>[2x]GSYDSSSSSSNDSSARNEEDESCMFALKLLGGFAVPFTIKAVIELGVMDQLLTAERAMSAEELVAAAVAAQLPRPEVACTMVDRLLRFLASHSVVRCTTEVVVGTDDATTTTCCRRSYAASPVCKWFARNGVEDSVLPLGMMILNKTFLDSWQNITDAVLEGAAPFEKTYGMPMFEYLSTNGPLNTVFHEAMANHSMIITKKLLKFFRGFEGLDVLVDVGGGNGTTLQMIRGQYKNMRGINYDLPHVIAQAAPVEGVEHVGGSMFDNIPRGNAVLLKWILHDWDDKACIKILKNCYTALHVRGKVIVLEYVVPDEPEPTLAAQGAFELDLTMLVTFGSGKERTQREFSELAMEAGFSREFKATYIFANVWALEFTK

A stilbene O-methyltransferase, SbSOMT, is first shown to be indispensable for pathogen-inducible pterostilbene (3,5-bis-O-methylated) biosynthesis in sorghum (Sorghum bicolor). Phylogenetic analysis indicates the recruitment of genus-specific SOMTs from canonical caffeic acid O-methyltransferases (COMTs) after the divergence of Sorghum spp. from Saccharum spp. In recombinant enzyme assays, SbSOMT and COMTs regioselectively catalyze O-methylation of stilbene A-ring and B-ring respectively. Whilst SbSOMT shows global structural resemblance to SbCOMT, molecular characterizations illustrate two hydrophobic residues (Ile144/Phe337) crucial for substrate binding orientation leading to 3,5-bis-O-methylations in the A-ring. The catalytic residues of SbSOMT are highly conserved with all reported COMTs, including His282 as the key nucleophile, whereas Asp283, Glu310, and Glu342 collectively charge the basicity or confine His282 in its reactive conformation.

To rationalize their different catalytic regioselectivities, structural analyses involving X-ray crystallography and computational methods were conducted. We solved the crystal structure of an SbSOMT-resveratrol-nicotinamide adenine dinucleotide (β-NAD) ternary complex (diffracted to 1.72 Å resolution, Fig. 4d; β-NAD was utilized as an additive to improve crystallization), an SbSOMT-resveratrol binary complex, and two ternary complexes reproduced with pinostilbene or pterostilbene (diffracted at 2.10 and 2.56 Å, respectively). All complexes were in high structural resemblance and depicted as a homodimer with an open conformation. Of the three hydroxyl groups on resveratrol capable of forming hydrogen bonds, only the methyl-accepting 3-OH group (A-ring) formed direct hydrogen bonds to SbSOMT residues, including the catalytic residues His282 (2.80 Å) and Asp283 (3.26 Å). The same binding mode was adopted for pinostilbene or pterostilbene in the corresponding SbSOMT co-crystals. Overall, these structures depicted a productive substrate orientation within the substrate binding pocket which greatly favors A-ring O-methylation. Meanwhile, SbSOMT also showed strong binding affinities towards resveratrol and pinostilbene (4.69 μM and 2.86 μM respectively) but a higher Kd to pterostilbene (11.20 μM), demonstrating SbSOMT favors its substrates over product for binding.>[2x]MAYDDLHEGYATYTGSGYSGGAFLLDPIPSDMEITAINPADLNYGGVKAALAGSYLEVEGPKGKTTVYVTD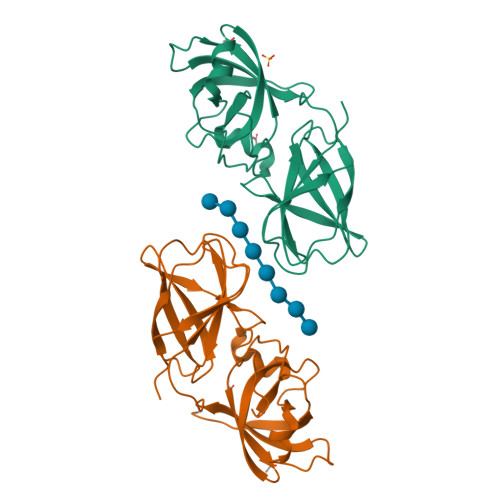LYPEGARGALDLSPNAFRKIGNMKDGKINIKWRVVKAPITGNFTYRIKEGSSRWWAAIQVRNHKYPVMKMEYEKDGKWINMEKMDYNHFVSTNLGTGSLKVRMTDIRGKVVKDTIPKLPESGTSKAYTVPGHVQFPE>[2x]GFTLPRQPTKAYECENCSQLSRENLHDKW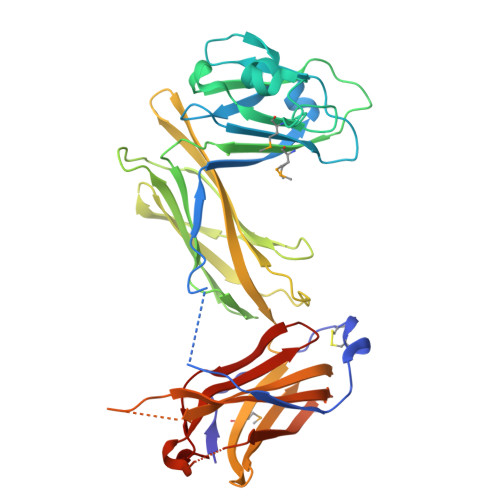EITNEPLNNNISNVRRSYGYKERISLEQLQRGVIISTLAPGAVVRITPLQNKSIPELLIKTPKNQLLPLKEASSLYNQDDEVGNNPLAITKHQAMLQIKPELGYGKFILKSKDITNKYADAYMISVLDKFSITYLEVETDSLHYQYGDKLKATISLHNDITEYDVNDVDARLVGPKGQVISLNLTKLKSNVFEGTATLDSELNDRGENWYLETDVQTEYGQEIIRRSGHTAFSYSIPSASLMNVKKLSSKPLTFVVTVDVATASRYALQSVLFQKNGKGEARPIQTSQRAQWLEPGKHVLQFTFDNHNQLSDDNLYLGYLRLIDYGQLKTVYQYNQPVKLSQLVD>[2x]AKPGPALWPLPLSVKMTPNLLHLAPENFYISHSPNSTAGPSCTLLEEAFRRYHGYIFGFYKWHHEPAEFQAKTQVQQLLVSITLQSECDAFPNISSDESYTLLVKEPVAVLKANRVWGALRGLETFSQLVYQDSYGTFTINESTIIDSPRFSHRGILIDTSRHYLPVKIILKTLDAMAFNKFNVLHWHIVDDQSFPYQSITFPELSNKGSYSLSHVYTPNDVRMVIEYARLRGIRVLPEFDTPGHTLSWGKGQK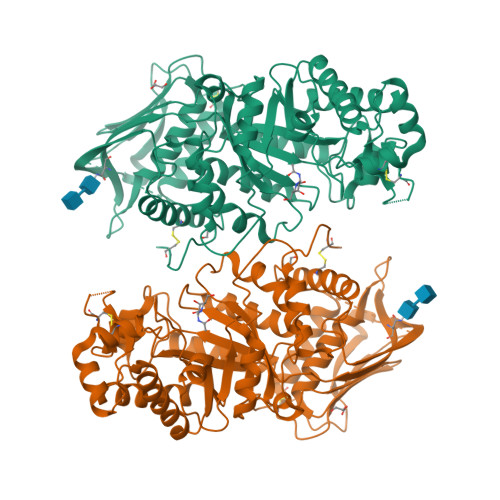DLLTPCYSRQNKLDSFGPINPTLNTTYSFLTTFFKEISEVFPDQFIHLGGDEVEFKCWESNPKIQDFMRQKGFGTDFKKLESFYIQKVLDIIATINKGSIVWQEVFDDKAKLAPGTIVEVWKDSAYPEELSRVTASGFPVILSAPWYLDLISYGQDWRKYYKVEPLDFGGTQKQKQLFIGGEACLWGEYVDATNLTPRLWPRASAVGERLWSSKDVRDMDDAYDRLTRHRCRMVERGIAAQPLYAGYCNHENM> MDETGKVLVLALYDYQEKSPREVTMKKGDILTLLNSTNKDWWKVEV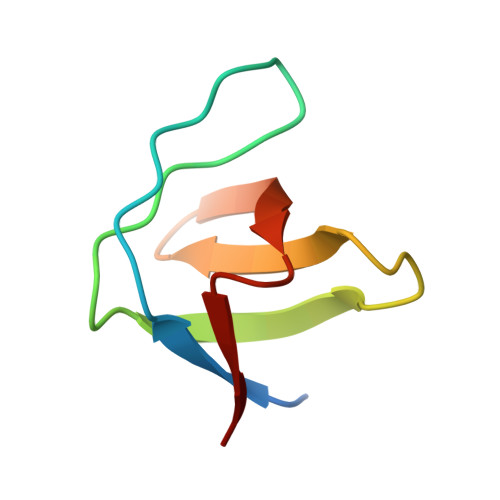NGRQGFVPAAYVKVL>MESTLGWSVQDWLSFHSKSTPTKSLELLENLLKSQKPAPEDPAWISLIPVEDLHHQWNILQSKSNKEELPLYGVPIAVKDNIDYKGLPTTAACPSYLYQPTRDSYVVELLRDAGAVVIGKTNLDQFATGLVGTRSPYGKTPCVFNDKYVSGGSSAGSASVVGRGIVPLSLGTDTAGSGRVPAALNNLIGLKPTKGAFSCRGVVPACKSLDCVSVFALNLSDAEIAFKVMNKPDLLEDEYSREFPKNPISQYPKDLTIAIPKEVPWFGETENPKLYTKAVASLKNTGAKIVVVDFEPLLELARCLYEGAWVAERYCATRDFLATNPPESSLDETVVNIIKGAVKFDAADAFKFEYKRQGILQKVNLLLKDIDVLCVPTCPLNPKLEEVAQEPVLVNSRQGTWTNFVNLADLAALAVPSGFRSDGLPNGITLIGKKFSDYALLDLAKRFFSVAFPNNSRTYGKFVDRRITVEDELDGPSKDTLNGVKLAVVGAHLKGLPLHWQLQKCNATYLSSPKTSNNYKLYALPKVGPVLKPGLRRVNDGTGSQIQLEVYSVPYDRFGDFIAMVPEPLGIGSVELESGEWVKSFICEEFGYTQQGTVDITKFGGFKPYIEHIQVTEAQKKKPFETVLIANRGEIAVRIMKTLKRMGIKSVAVYSDPDKYSQHVTDADFSVALHGRTAAETYLDIDKIINAAKKTGAQAIIPGYGFLSENADFSDRCSQENIVFVGPSGDAIRKLGLKHSAREIAERAKVPLVPGSGLIKDAKEAKEVAKKLEYPVMVKSTAGGGGIGLQKVDSEDDIERVFETVQHQGKSYFGDAGVFMERFVNNARHVEIQMMGDGFGKAIAIGERDCSLQRRNQKVIEETPAPNLPEATRAKMRAASERLGSLLKYKCAGTVEFIYDEQRDEFYFLEVNARLQVEHPITEMVTGLDLVEWMLRIAANDSPDFDNTKIEVSGASIEARLYAENPVKDFRPSPGQLTSVSFPSWARVDTWVKKGTNVSAEYDPTLAKIIVHGKDRNDAIMKLNQALNETAVYGCITNIDYLRSIASSKMFKEAKVATKVLDSFDYKPCAFEVLAPGANTSVQDYPGRTGYWRIGVPPSGPMDSYSFRLANRVVGNNSKSPALEITLNGPKLLFHTETVIAVSGGTVSCTLNDAQIAQNEPIEVKRGDILSVGKVTVGCR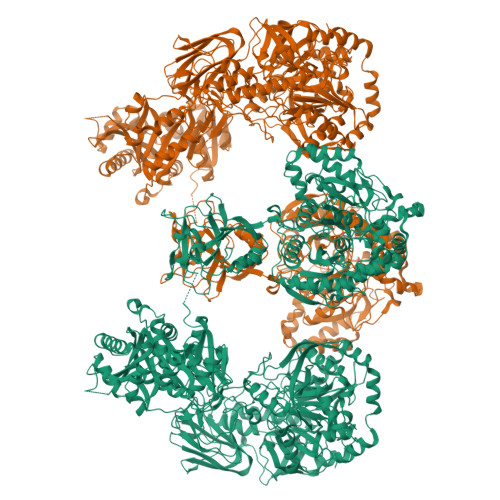AYLSIRGGIDVPEYLGSRSTFAMGNMGGYNGRILKLGDVLFLNQPELSVSSLPAPDFEPQAAPKSLLPTLSTNKDWKIGVTCGPHGSIDLFKEEYIEQFFNDKWKVHYNSNRFGVRLIGPKPKWARSDGGEAGLHPSNAHDYVYSLGAINFTGDEPVIITCDGPSLGGFVCQAVVAEAELWKVGQLTPGDTIQFVPLSYGVARQLKESQDKSIDNFEEGSLLELSDDKILPKYENPILAVLPKKSDLSPKVTYRQAGDRYILVEYGELEFDLNICYRINRLIHQVERHQTVGIVEMSQGVRSVLIEFDGSKINQKALLKCLIAYESEIQFDKNWNVKSKIFKLPMAFEDSKTLDCVTRYRETIRSEAPWLPNNVDFIADVNDIDRNDVKNMLYSAKFMVLGLGDVFLGSPCAVPLDPRHRYLGTKYNPSRTYTARGVVGIGGMYMCIYNAEGSPGGYQLVGRTITAWDKLVIGDHPIDHPWLLTPFDQVEFYPVTEEELEVIIEDNDNGKFKIDVEESIFDHKEYLAWINENIDSIVAFQEAQGGEKADEFARLIQVANAELKKSGDDKPQDVEEYPDDAELLYSEYTGRFWKPVAAVGDHVEAGDGVIIIEAMKTEMVVGATKSGKVYKILHKNGDMVEAGDLVAVIV[4x]>GPGSEFMDEKTKKAEEMALSLTRAVAGGDEQVAMKCAIW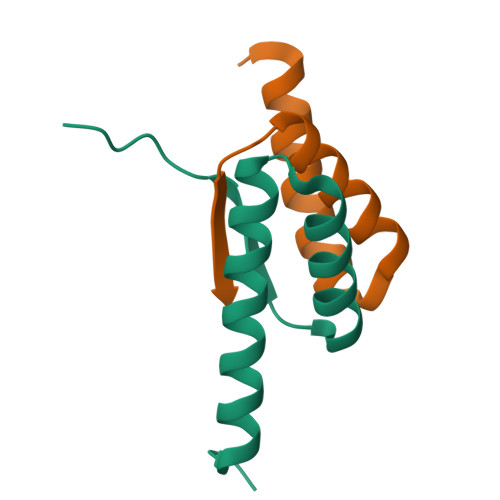LAEQRVPLSVQLKPEVSP[4x]> PKCMIFCPVAATPAQQDALLKDAEKAVADALGKPLSYVMVGYSQTGQMRFGGSSDPCAFIRVASIGGITSSTNCKIAAALSAACERHLGVPKNRIYTTFTNKSPSEWAMGDRTF

Macrophage migration inhibitory factor (MIF) is a proinflammatory molecule in mammals that, unusually for a cytokine, exhibits tautomerase and oxidoreductase enzymatic activities. Significantly, homologues of MIF have been described in many parasitic species including Plasmodium, Leishmania, Brugia, Clostridium, and Eimeria, and it has been implied that these proteins facilitate the manipulation of the host immune response during infection. Herein, we produced recombinant histidine-tagged Toxoplasma gondii MIF (TgMIF), a 12-kDa protein that lacks oxidoreductase activity but exhibits tautomerase activity with a specific activity of 19.3 μmol/min/mg that cannot be inhibited by the human MIF inhibitor ISO-1. We also demonstrate that TgMIF can elicit IL-8 production from human peripheral blood mononuclear cells while also activating ERK MAPK pathways in murine bone marrow-derived macrophages.

The crystal structure of the TgMIF homotrimer has been determined to 1.82 Å, and although it has close structural homology with mammalian MIFs, it has critical differences in the tautomerase active site that account for the different inhibitor sensitivity. Crystals formed in space group H3(2) and x-ray diffraction data were collected at the Diamond Light Source. TgMIF forms a crystallographic trimer, and each monomer consists of a four-stranded mixed β-sheet and two α-helices stacked against a β-sheet. The topology of the TgMIF trimer (a ring with a central pore, coincident with the molecular 3-fold axis) is conserved with HsMIF as seen in superimposition images. Second, Pro15, which is conserved in mammalian MIFs and functions as a helix “breaker” between the η1 turn and α1 helix in HsMIF, is substituted with Glu16 in TgMIF. As a result, the α1 helix in TgMIF is longer than in HsMIF, extending from Pro13 to Leu31. Third, the central pore of the TgMIF trimer is narrower than that of mammalian MIFs with a minimum pore diameter of 3.5 Å at Arg61. Moreover, three sulfate ions were bound to positively charged residues lining the pore, notably Arg61 and Lys2, as well as a network of water molecules. However, replacement of Asn97 for Thr98 in the TgMIF tautomerase active site is of importance as this substitution prevents the formation of a hydrogen bond between MIF and the substrate molecule, l-DOPA methyl ester. Further substitutions around the TgMIF tautomerase active site are observed whereby Val106 is replaced by Trp107, resulting in possible steric hindrance that prevents the successful binding of ISO-1 to the active site.> EPTAEMLANNCAGCHGTR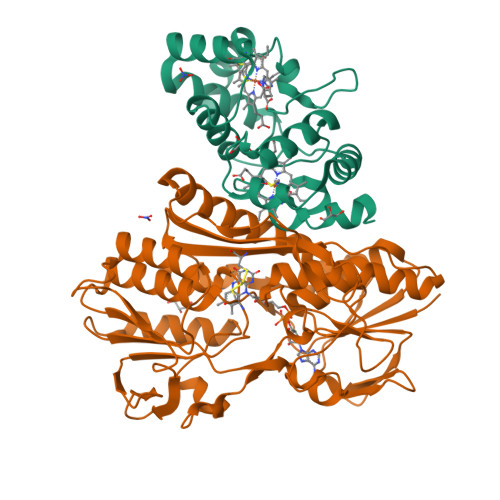GNSAGPASPSIAQMDPAVFVEVMEQFKSGEIQSTIMGRIAKGYSTADFQKMAEYFKQQTYQPVKQSFDKALVAKGTKLHDKYCEKCHVESGKPLADQDEYHILAGQWTPYLRYAIEDFRAERRPMEKKMASKLKELLKAEGEDGLDALFAFYASQQ;> AGRKVVVVGGGTGGATAAKYIKLADPSIEVTLIEPNETYYTCYMSNEVIGGDRELASLRVGYDGLRAHGIQVVHDSALGIDPDKKLVKTAGGAEFAYDRCVVAPGIDLLYDKIEGYSEALAAKLPHAWKAGEQTALLRRQLESMDDGGVVIIAPPAPPFRCPPGPYERASQIAHYLKAHKSKSKVIILDNSQTFSKQAQFTKGWERLYGFGTENALIEWHPGPDAAVVKTDTEAMTVETSFGETFKAAVINLIPPQRAGKIAQSASLTNDSGWCPVDIRTFESSLQPGIHVIGDACNAAPMPKSAYSANSQAKVAAAAVVALLKGEEPGTPSYLNTCYSILAPGYGISIAAVYRPNAEGKAIEAVPDSGGITPVDAPDWVLEREVQYAHSWYNNIVHDTFG>GPLGSEQKKMKYLENLVGKTPM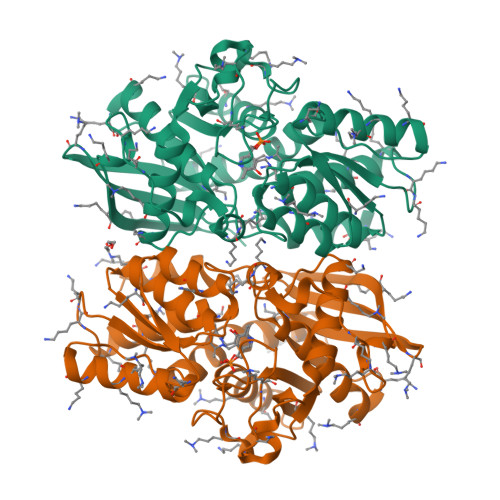LELIFDYKGEERRIFVKNESYNLTGSIKDRMAFYTLKKAYEKNEIKKGAPIVEATSGNTGIAFSAMGAILGHPVIIYMPDWMSEERKSLIRSFGAKIILVSRKEGGFLGSIEKTKEFAKNNPDTYLPSQFSNLYNSEAHYYGIGLEIVNEMKSLNLNIDGFVAGVGTGGTVMGIGKRIKENFSNAKICPLEPLNSPTLSTGYKVAKHRIEGISNEFIPDLVKLDKLDNVVSVDDGDAIVMAQKLAKCGLGVGISSGANFIGALMLQNKLGKDSVIVTVFPDDNKKYLSTDLMREEKVKEDFLSKDITLKEIKNVLRVI[2x]> GPLGSGGGTIAMLNEISSDTLEQLYSLAFNQYQSGKYEDAHKVFQALCVLDHYDSRFFLGLGACRQAMGQYDLAIHSYEEGAVMDIKEPRFPFHAAECLLQKGELAEAESGLFLAQELIANKPEFKELSTRVSSMLEAIKLKKEMKH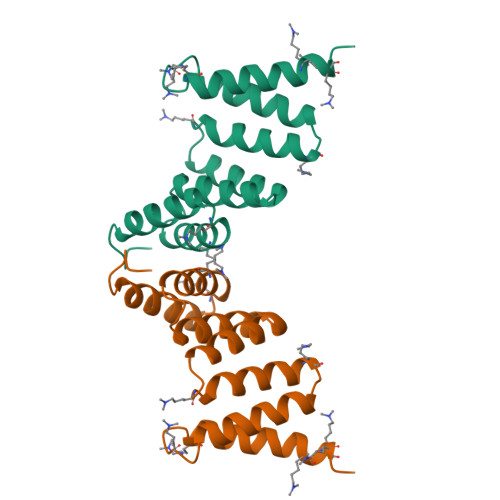E>TDENLKIAIASSPAPRYITDMSIEEISREWYMLMPRQKITGGLMVKMDQAIMDKRITLKANFSVLFDQLETLVSLRAFTDDGAIVAEISPIPSMPGHSTEDVKNAIGILIGGLEWNDNSIRASENIQRFAWGIRDENGGPPLPPK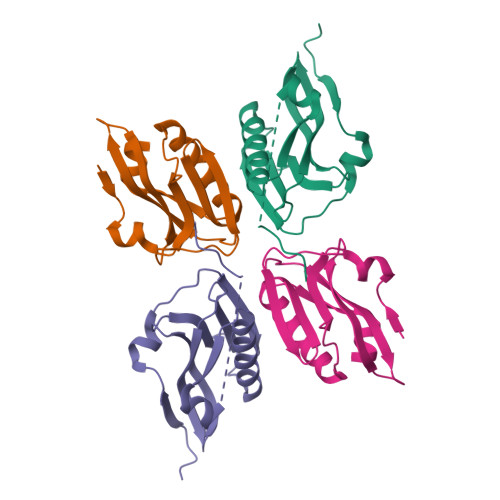QKRYMARRVESEV[2x]>HMVNGKVALVTGAAQGIGRAFAEALLLKGAKVALVDWNLEAGVQCKAALDEQFEPQKTLFIQCDVADQQQLRDTFRKVVDHFGRLDILVNNAGVNNEKNWEKTLQINLVSVISGTYLGLDYMSKQNGGEGGIIINMSSLAGLMPVAQQPVYCASKHGIVGFTRSAALAANLMNSGVRLNAICPGFVNTAILESIEKEENMGQYIEYKDHIKDMIKYYGILDPPLIANGLITLIEDDALNGAIMKITTSKGIHFQDY[2x]

The enzyme 15-prostaglandin dehydrogenase (15-PGDH) is a key negative regulator of tissue stem cell activity in proliferation and in the repair of tissue injury, whose negative regulation of tissue regeneration is conserved across multiple organs. 15-PGDH acts via its NAD+-dependent enzymatic activity of oxidizing and degrading prostaglandin E2 (PGE2), and related eicosanoids, which provide key trophic support for stem cells in multiple tissues. Specifically, 15-PGDH catalyzes the rate-limiting step to initiate PGE2 degradation by oxidizing the 15-hydroxyl moiety of PGE2 to a 15-keto group, thereby inactivating PGE2 from being able to bind to its receptors. 15-PGDH assembled as a homodimer, which is the proposed physiological form of the enzyme.

To gain insight into the molecular details of 15-PGDH inhibition, we used cryo-EM and single-particle analysis to solve the structure of the human 15-PGDH protein bound to (+)-SW209415, a second-generation 15-PGDH inhibitor, plus the NADH cofactor. Despite the relatively small size of the monomeric protein (29 kDa), image and post-processing yielded a cryo-EM map for the 15-PGDH-SW209415-NADH complex at a nominal resolution of 2.4 Å. Following asymmetric refinement, the cryo-EM structure exhibits strong density for (+)-SW209415 in a well-defined binding pocket in each of the 15-PGDH protomers. Strikingly, (+)-SW209415 is buried within the 15-PGDH protein with molecular contacts formed on all sides of the inhibitor. Cumulatively, the interaction of the sulfoxide of the inhibitor with S138 and Y151 of 15-PGDH contributes significant binding energies and so serves to coordinate (+)-SW209415 interactions with 15-PGDH. The thienopyridine moiety of (+)-SW209415 is sandwiched between F185 and L139, where π-stacking with F185 provides the largest contribution of all 15-PGDH residues in binding energy. The thienopyridine reaches into the catalytic pocket where an amine group at position 3 forms a hydrogen bond with Q148 of 15-PGDH. Additionally, the (+)-SW209415 thiazole contributes to binding through π-stacking interactions with Y217 and hydrophobic interactions with L139 of 15-PGDH. Finally, while not as well resolved in the cryo-EM density, the butyl chain of (+)-SW209415 occupies a hydrophobic pocket that is surrounded by I190, L191, and I194 of 15-PGDH. Thus, the MD simulations recapitulate the cryo-EM findings that the lid becomes disordered in the absence of inhibitor binding. Together these results show that binding of (+)-SW209415 stabilizes the lid structure of the α10-α12 triple-helix to create a stable configuration of (+)-SW209415 complexed with 15-PGDH.> GSSGSSGMNLLSQVSFWVGCGILAFGSIVFGLGAWNAKRQSWEEFYIVHFTVTTVAACAYLAMAMGQGEITLQNTDLAAEGVRHIYWARYCDWIVTTPLILFSICRLSKVRGTMIAGIIMSDVLMIITGAIAAFSFAPERYVWYIVSCMFEVAIFVILLGAVRTSAMRQHYDVKNLFNLVFTVFSIYFWAYPIVWILGQKGVGLYGTGVESLLIMLLDITAKVFYGFLLLRDRETLQRMGQLSSVPNSGSGVGNYR

Rhodopsin is a photoreceptor membrane protein that binds retinal as the sole chromophore, a simpler light-utilizing system than the chlorophyll-based photosystem, which consists of many proteins and typically multiple chromophores. Here, we used a metagenomic mining approach, which led to the identification of a novel rhodopsin clade unique to cyanobacteria, cyanorhodopsin-II (CyR-II). CyR-IIs function as light-driven outward H+ pumps. The CyR-II clade is further divided into two subclades, YCyR-II and GCyR-II, based on their specific absorption wavelength.

The crystal structure of cell-free-synthesized P7104R was solved at 2.07 Å to clarify the red-shifted absorption mechanism of P7104R. The P7104R monomer was composed of seven transmembrane helices (helices A–G) as well as other rhodopsins. A detailed comparison between the structure of P7104R and N2098R or BR showed that a pentagonal cluster near the retinal of P7104R, which is known to be important for proton transport, consisted of three water molecules adjacent to the Lys215P7104R, Asp85P7104R, and Asp211P7104R (corresponding to Lys216BR, Asp85BR, and Asp212BR). The structure around the proton exit was also similar in arrangement, although Glu (Glu182N2098R and Glu194BR) was replaced by Lys193P7104R. The cyclohexane ring comprising the retinal chromophore of P7104R was more slanted than those of N2098R and BR. A comparison of the amino acids around the retinal showed that the Ile171N2098R was rearranged to a Trp182P7104R containing a larger functional group, and the distorted structure of the retinal was canceled by Trp182P7104R, through Phe181P7104R and Glu144P7104R (orange bold). The F181W, W182I, and F181W/W182I mutants of P7104R absorbed at wavelengths of 565.0, 565.5, and 557.5 nm, respectively, which were blue-shifted compared with the wild type of P7104R (λmax = 570 nm). These results provide support for the hypothesis and indicate that Phe181P7104R and Trp182P7104R play a role in the red-shift of the absorption maximum in YCyR-IIs. Through our structural analysis, the high pKa value in P7104R may also be stabilized via a hydrogen bond between Ser96P7104R and His42P7104R.>MAAGLTTRNIEHAVIQVREENKFSLLKDVLMTENPDSCIIFCRTKEHVNQLTDELDDLGYPCDKIHGGMIQEDRFDVMNEFKRGEYRYLVATDVAARGIDIENISLVINYDLPLEKESYVHRTGRTGRAGN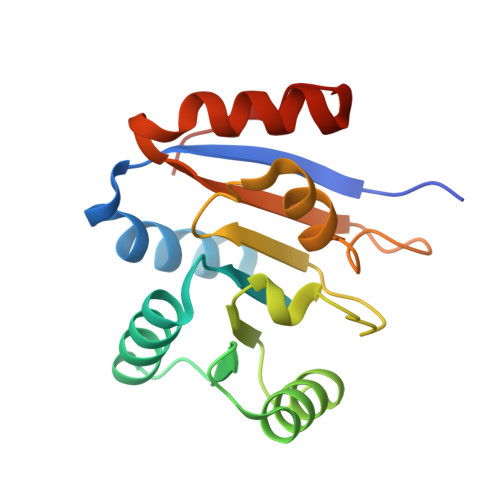KGKAISFVTAFEKRFLADIEEYIGFEIQKIEA[2x]>MNHHYRDTRKIDPSRGATLGDGTPNDNDRIEIGPTQLAFSEWAAAGLQLPNLDRMREYRWKRLTQAIVDRGYGGLLMFDPLNIRYATDSTNMQLWNTHNPFRAVLLCADGYMVIWDYKNSPFLSKFNPLVREQRSGADLFYFDRGDKVDVQADVFANEVRVLMQDHAPGHTRLAVDKIMLHGLRALEAQGFEIMEGEEVTEKTRAIKGPDEILAMRCASHACETAVAEMEKFARAHVGDGKTSEDDIWAVLHAENIKRGGEWIETRLLASGPRTNPWFQECGPRITQKNEIIAFDTDLIGSYGICVDISRTWWIGDQKPRPDMVYAMQHAHEHIMTNMEMLKPGVMIPDLTANCHRLDDKFQAQKYGCLMHGVGLCNEWPLVAYPDKAVPGSYDYPLEPGMVLCVEAAVGEVGGDFSIKLEDQVLIT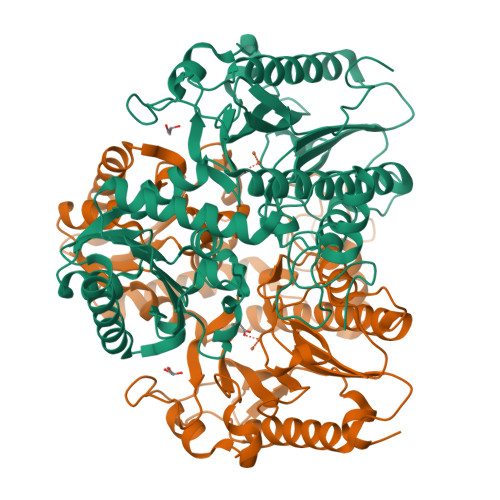EDGYENLTTYPFDAALMGLA[4x]The R2TP complex is found in organisms from yeast to humans, and consists of the AAA+ ATPases Rvb1 and Rvb2 (human: RUVBL1 and RUVBL2), a TPR-containing protein, Tah1 (human: Spagh or RPAP3), and Pih1 (also known as NOP17 and Pih1D1, but referred to as Pih1 henceforth; Kakihara and Houry, 2012; Te et al., 2007). Pih1 is the multipoint scaffold of the R2TP complex, coupling the Rvb1-Rvb2 hetero-dodecamer, the Hsp90 chaperone machinery (via Tah1 in yeast or Spagh/RPAP3 in metazoa), and the TTT (Tel2-Tti1-Tti2) complex implicated in activation and stabilization of PIKKs (Hurov et al., 2010; Kakihara and Houry, 2012). The biological roles ascribed to the R2TP complex are directly associated with its ability to interact with the Hsp90 chaperone system and function as an Hsp90 cochaperone (Boulon et al., 2010; Izumi et al., 2012; Takai et al., 2010). Here we present crystal structures of Hsp90-Tah1-Pih1, Hsp90-Spagh/RPAP3, and Pih1-Tel2 complexes that together define key structural links within the R2TP core in yeast and in animals and reveal how R2TP connects the Hsp90 chaperone system to the TTT complex involved in PIKK activation.

We next determined the crystal structures of each of the TPR domains (TPR1 and 2) of human Spagh/RPAP3 cocrystallized with the Hsp90 C-terminal peptide. Spagh-TPR2267–381 consists of six α helices, with the first five again aligning with Tah1-TPR. The N-terminal helix of Spagh-TPR2 is double the length of the N-terminal helices of Tah1 or Spagh-TPR1 and projects out of the core TPR domain. In both Spagh/RPAP3 TPR domains, the Hsp90 C-terminal peptide is bound in the groove formed by the first five α helices. The peptide bound to TPR2 adopts a compacted conformation very similar to the Tah1 complex, making extensive interactions with the walls of the groove. The Hsp90 peptide bound to TPR1 makes fewer interactions and is less well structured, but in both cases the α-carboxyl and the side chain of the C-terminal aspartic acid are bound by a “carboxylate clamp” (Scheufler et al., 2000), anchored by the side chains of Asn 172 (TPR1) and Asn 321 (TPR2), each of which make a bidentate interaction with the peptide NH and α-carboxyl of the C-terminal aspartic acid residue of the Hsp90 peptide. The TPR1 and TPR2 domains of Spagh/RPAP3 have a typical TPR domain structure, but lack the distinct hydrophobic pocket formed between helices 5 and 7, into which the methionine side chain of the MEEVD motif binds (Morgan et al., 2012; Zhang et al., 2005). Instead and similar to Tah1, the methionine side chain packs against the surface of helix 5 and remains partially exposed. Mutation of TPR1 (N172E) or TPR2 (N321E) and fitting with a two site model suggested that binding for one site (nonmutant site) remained unaffected (N172E-TPR1 mutant, TPR2: KD = 9.7 μM and N321E-TPR2 mutant, TPR1: KD = 0.94 μM), whereas the mutated TPR sites were compromised for binding (N172E-TPR1 mutant, TPR1: KD = ∼231 μM and N321E-TPR2 mutant, TPR2: KD = ∼109 μM).

>[2x]STEGERKQIEAQQNKQQAISEKDRGNGFFKEGKYERAIECYTRGIAADGANALLPANRAMAYLKIQKYEEAEKDCTQAILLDGSYSKAFARRGTARTFLGKLNEAKQDFETVLLLEP;>[2x]SRMEEVD> TFNMELYNTDLFLVPSPGVFSVAENEHV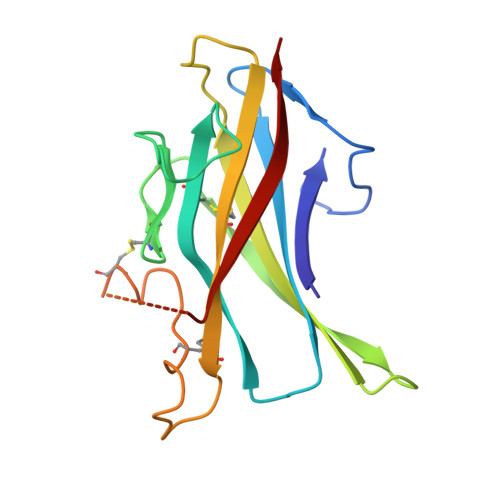YVEVSVTKADQDLGFAIQTCFISPYSNPDRMSDYTIIENICPKDDSVKFYSSKRVHFPIPHAEVDKKRFSFVFKSVFNTSLLFLHCELTLCSRNKGSQKLPKCVTPDDACTSLDATMIWTMMQNKKTFTKPLAVVLQVD Here we characterize the MerR-type transcriptional regulator Alr3614 that is encoded by one of the CAST (AnCAST) system genes in the genome of cyanobacterium Anabaena sp. PCC 7120. Alr3614/CvkR is translated from leaderless mRNA and represses the AnCAST core modules cas12k and tnsB directly, and indirectly the abundance of the tracr-CRISPR RNA. We identify a widely conserved CvkR binding motif 5’-AnnACATnATGTnnT-3’. CvkR repressors are at the core of a widely conserved regulatory mechanism that controls type V-K CAST systems.

To investigate CvkR functionality at the structural level, a high-quality crystal structure was determined at 1.6 Å resolution. CvkR consists of a classical winged helix-turn-helix (wHTH) DNA-binding domain at the N-terminus (residues 1-80), a dimerization domain (residues 81-132), and a potential effector-binding helix in the C-terminal region (helix α7, residues 133-150), in which an ATP, used as reagent for optimal crystal formation, was bound as a ligand. By dynamic light scattering (DLS), a ~5.1 nm (~51 Å) average diameter was measured for CvkR, consistent with its assembly into a homodimer of ~54 Å in the solved crystal structure and the result of our SEC analysis. Three antiparallel β-strands (β2-β1-β3) and one short α-helix (α6), together with the equivalent β-strands and helix of the other subunit, comprise the bulk of the dimerization interface. The contacts are predominantly hydrophobic and bury 997.6 Å2 surface area (PDBePISA)47, which is much smaller than that observed in canonical MerR-type proteins, for instance, 1896.8 Å2 in CueR. In comparison, the mode of CvkR dimerization significantly differs from MerR-type regulators such as CueR39 or MtaN48, which assemble into homodimers via two-helix antiparallel coiled-coil (α5/α5’), and is also distinct from the unusual MerR-type TnrA/GlnR family regulators, which form homodimers relying on an N-terminal extra helix (e-α1/e-α1’). Therefore, the pattern of CvkR dimerization is unique among the MerR family members. In our solved structure, the crystal optimizing reagent ATP was bound near the putative effector binding site through π–π stacking, cation–π, and several hydrogen bonds. While the nonspecific hydrogen bonds at the N1 and N6 positions of the adenine moiety, together with the unbound triphosphate group in the putative effector binding site, suggest that ATP is not the natural effector of CvkR, other nucleoside derivatives might be possible candidates. However, subsequent EMSA experiments showed no effects on CvkR DNA binding when such ligands were added, indicating that ATP and its analogs are indeed not the natural effectors of CvkR.

> HMGSMEGKFYTSTEASEITHCSRRQLQYWREKGVIVPTVNSSGKGRNVYYSKADLLALTVMEQLLSTGLNFDLCYAALQTLRKQEPWLFDESVPEEKMKRLMLLPTRSPEQPLQLAEFDKQAALEALCHGQTVIPFWSDRIHQQLRENLKSFSS>MAGKSPEEEHPVKAYGWAVKDRTTGILSPFKFSRRATGDNDIRIKILYCGICHTDLTSVKNEYEFLSYPLVPGMEIVGIATEVGSKVTKIKVGEKVAVAAYLGTCGKCYNCVNDLENYCPEVIIGYGTPYHDGTINYGGLSNETVVNERFVLRFPEKLSPAGGAPLLSAGITAYSAMRNHGLDKPGIHLGVVGLGGLGHLAVKFAKAFGVRVTVISTTPSKKDEAINNLGADAFLFSRDDKQMRAAIGTFDAIIDTLAVVHPIAPLLDLLRSHGKLVLVGAPSKPLELPTIPLLSGGKSLIGSAAGNVKQTQEMLDFAAEHDITANIEVIPIDYINTAMERLDKGDIRFRFVVDIENTLTPPPEP[2x]

pmcAlcohol dehydrogenases (ADHs EC 1.1.1.1) are NAD(P)H‐dependent medium‐chain oxidoreductases found in all kingdoms of life. These enzymes typically catalyse the reversible reduction of aldehydes or ketones to the corresponding alcohol. The structural motifs of ADHs are highly conserved in all known eukaryotic examples; most notably, a zinc ion involved in catalysis, a second zinc ion involved in maintaining protein structure, and the Rossmann peptide‐fold involved in cofactor binding. ADHs have been shown to catalyse many complex biochemical transformations in plant natural product biosynthesis, suggesting that their catalytic repertoire has been expanded.

Here we report the crystal structure of dihydroprecondylocarpine acetate synthase (DPAS), an ADH that catalyses the non‐canonical 1,4‐reduction of an α,β‐unsaturated iminium moiety. We report four crystal structures of apo‐ and substrate‐bound DPAS from two phylogenetically related species. These structures reveal, surprisingly, the loss of the catalytic zinc ion from the DPAS active site, indicating that zinc is not strictly required for reduction by ADHs. Despite the presence of NADP+ in DPAS crystallisation conditions, none of the solved structures had sufficient density to model the cofactor. Although electron density for the structural zinc ion was clearly observed in all TiDPAS2 structures (the CrDPAS structure lacked electron density for this region), surprisingly, the substrate pocket lacked electron density at the expected site of the catalytic zinc. The lack of the catalytic zinc in DPAS is substantiated by the observation that two of the conserved catalytic zinc coordinating residues are mutated (His74Met and Cys168Ser). Computational estimation found TiDPAS2 had a larger substrate cavity than other structures of ADHs involved in monoterpene indole alkaloid (MIA) biosynthesis.>[4x]MSFRFGQCLIKPSVVFLKTELSFALVNRKPVVPGHVLVCPLRPVERFHDLRPDEVADLFQTTQRVGTVVEKHFHG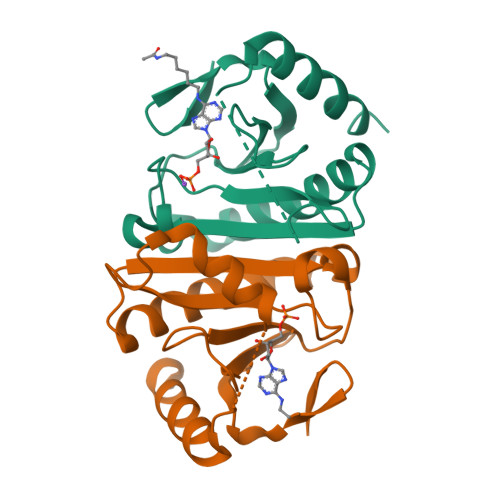TSLTFSMQDGPEAGQTVKHVNVHVLPRKAGDFHRNDSIYEELQKHDKEDFPASWRSEEEMAAEAAALRVYFQHHHHHHAAWSQAQFEK N~2~-[(6-chloronaphthalen-2-yl)sulfonyl]-N~2~-{(3S)-1-[(2S)-1-(4-methyl-1,4-diazepan-1-yl)-1-oxopropan-2-yl]-2-oxopyrrolidin-3-yl}glycinamide 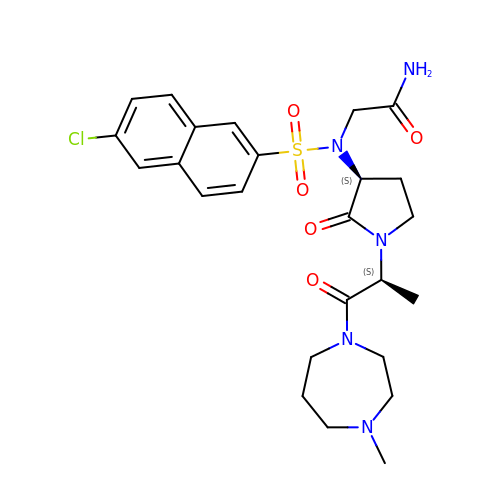| C25 H32 Cl N5 O5 S | JZNNJFBGWSQFIG-JTSKRJEESA-N>MADGGRVAQARALLQQCLHARLQVRPADGDAAAQWVEIRRGLVIYVCFF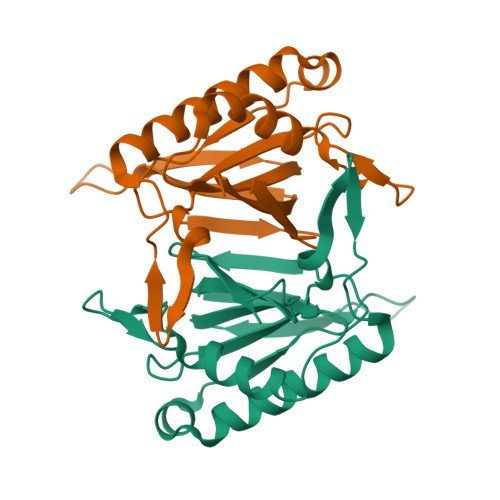KGADTDLLPKMVNTLLNVKLSETETGKHVSILDLPGDVLIIPQATLGGRVKGRSMQYHSNSGKEEGSELYSQFVSLCEKAVANNTKSVEAGVAVAHGTYGNRQVLKLDTNGPYTHLIEF[2x]> QQSCNTPSNRACWTDGYDINTDYEVDSPDTGVVRPYTLTLTEVDNWTGPDGVVKEKVMLVNNSIIGPTIFADWGDTIQVTVINNLETNGTSIHWHGLHQKGTNLHDGANGITECPIPPKGGRKVYRFKAQQYGTSWYHSHFSAQYGNGVVGAIQINGPASLPYDTDLGVFPISDYYYSSADELVELTKNSGAPFSDNVLFNGTAKHPETGEGEYANVTLTPGRRHRLRLINTSVENHFQVSLVNHTMTIIAADMVPVNAMTVDSLFLGVGQRYDVVIEASRTPGNYWFNVTFGGGLLCGGSRNPYPAAIFHYAGAPGGPPTDEGKAPVDHNCLDLPNLKPVVARDVPLSGFAKRPDNTLDVTLDTTGTPLFVWKVNGSAINIDWGRPVVDYVLTQNTSFPPGYNIVEVNGADQWSYWLIENDPGAPFTLPHPMHLHGHDFYVLGRSPDESPASNERHVFDPARDAGLLSGANPVRRDVTMLPAFGWVVLAFRADNPGAWLFHCHIAWHVSGGLGVVYLERADDLRGAVSDADADDLDRLCADWRRYWPTNPYPKSDSGL

Laccases (E.C. 1.10.3.2) possess a great biotechnological potential due to their ability to oxidize a wide range of phenolic substrates, spanning from small toxic phenols to large biopolymers such as lignocellulose. Like other multicopper oxidases, laccases operate via catalytic Cu-centers and coupling of the oxidative reaction to reductive cleavage of atmospheric oxygen into water. The overall fold of the three domain laccases consists of three cupredoxin-like domains with the catalytic copper sites located at domain 3 (C) and the trinuclear copper centre located at the interfaces between domain 1 (A) and 3 (C). The catalytic centres comprise three distinct types of copper ions classified by their spectroscopic properties, an electron shuttling Type 1 Cu (T1), and a trinuclear copper cluster (TNC) formed by a mononuclear Type 2 Cu and a binuclear Type 3 Cu site.

With the aim of elucidating the structure and function of asco-laccases, we have undertaken the structure determination of the asco-laccase from the thermophilic fungus Myceliophthora thermophila (MtL), The structure is known of four other asco-laccases (AA1_3): MaL from Melanocarpus albomyces, TaL from Thielavia arenaria, BaL from Botrytis aclada and AnL from Aspergillus niger. MtL crystallizes in space group C2221 with one molecule per asymmetric unit. In the crystal, N-linked glycosylation could be seen at seven out of ten consensus sites (N-x-T/S). Additional difference electron density was interpreted as two Ca2+ ions originating from the crystallization conditions. One of these (CA605) is directly involved in crystal packing mediating contacts between two symmetry related molecules as it coordinates to Asp530 and Asp534 in one molecule and the carbonyl oxygen of Val341 in another molecule. The MtL structure contains three fully occupied copper ions in the TNC-site. The site was modelled as a classical resting state with oxidized Cu ions, a hydroxide ion bridging the T3-coppers and a water/hydroxide ion coordinated to the T2-Cu, as this appeared to be the major component present. In the MtL structure, the T1-pocket is devoid of any ligands, buffer components or cryo reagents. The MtL protomers are related by a twofold crystallographic symmetry axis parallel to b, show significant shape complementarity and a larger buried surface area than the MaL and TaL dimers, but similar to the BaL dimer. The regions forming the dimer interface have low sequence conservation. It is interesting that the interface contains most of the loops that creates the T1-pocket of the MtL structure, which is sealed by the dimer formation, allowing access only via a conserved narrow solvent channel.>MSLAPCGLVPSARQLEWYNREMIAFFHFGINTFEEYVNEGDGKASTAIFNPTALDCRQWMQTLKAAGIPAAILTAKHADGFCLWPSKYTDYSVKNAAWKNGKGDVVREFVDACEEYGLKAGIYLGPHDRHEHLSPLYTTERYKEYYAHQLGELMSDYGKIWETWWDGAGADELTTPVYRHWYKIVREKQPDCVIFGTKNSYPFADVRWMGNEAGEAGDPCWATTDSVAIRDEAQYYKGLNEGMLDGDAYIPAETDVSIR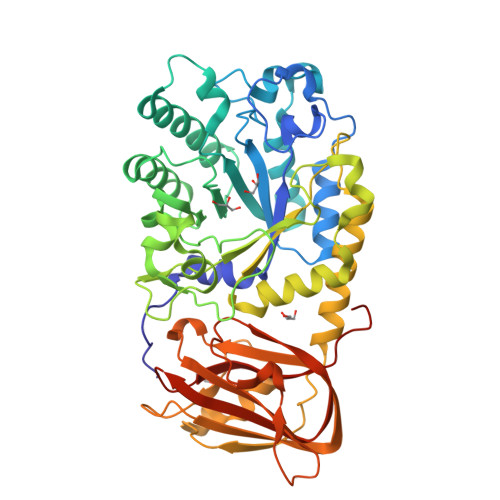PSWFYHAEEDSRVKSVRELWDIYCTSVGRNSVLLLNFPPDRRGLIHSTDSLHAALLKQGIDETFSTNLLRGAKVKATNVRGAKYSPEKMLDNEKNTYFAGKDGEVKADIIFTLPKTIEFDCLMIEEVIELGHRTTKWSVEYTVDGKNWITIPEATDKQAIGHKWIVRLAPVKAKQVRLRIQDGKACPAIHTFGVYKQSPVFKEGHHHHHH[2x]>MVMLSNFIAPDSNDPRLRIKSRYQMLVDGKSVDAASGSTIDRVSPGHAGEVVGTWPEASADDVRKAVAAARKAFDAGPWPRMSGAERSRLMFKVADLILARQEELALIESLEVGKPIAQARGEIGFCADLWSYAAGQARALEGQTHNNIGDDRLGLVLREPVGVVGIITPWNFPFIIASERVPWAIGSGCTVVLKPSEFTSGTSIRLAELAREAGIPDGVFNVVTGYGDPAGQVLAEDPNVDMVAFTGSVRVGTKLGEIAARTVKRVGLELGGKGPQIVFADADLDAAADGIAYGVYHNAGQCCISGSRLLVQEGIRDALMERLLDISRKVAFGDPLNERTKIGAMISEAHAEKVHSYVTAGITSGAELLLGGERIGREAGLYYAPTVFAGVTPDMSIAREEIFGPVLSTLTFKTADEAVALANATEFGLSASVWSTNLETALQTIR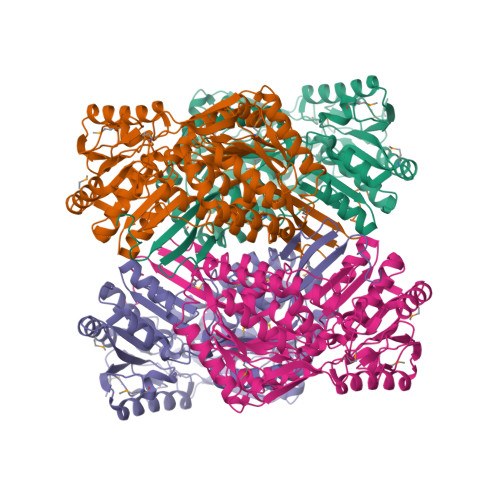RIRAGRCWINSVIDGTPELPIGGYKKSGLGRELGRYGFDEYSQFKGVHVTLGRPAPWFTAENLYFQSHHHHHHWSHPQFEK[4x]[(2R,5S)-5-(4-amino-5-fluoro-2-oxopyrimidin-1(2H)-yl)-1,3-oxathiolan-2-yl]methyl 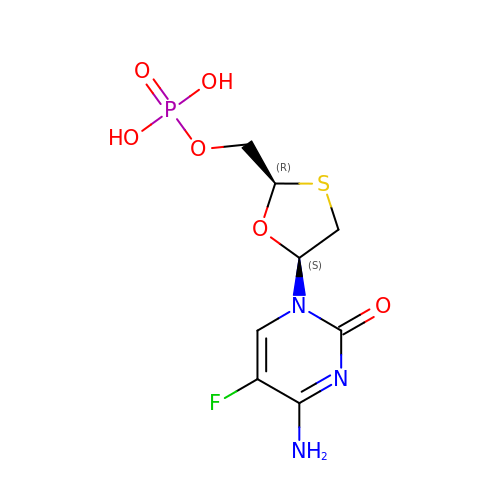dihydrogen phosphate | C8 H11 F N3 O6 P S | WQOMZMVXTRGMHZ-NTSWFWBYSA-N>MHHHHHHEPLILTAAITGAETTRADQPNLPITPEEQAKEAKACFEAGARVIHLHIREDDGRPSQRLDRFQEAISAIREVVPEIIIQISTGGAVGESFDKRLAPLALKPEMA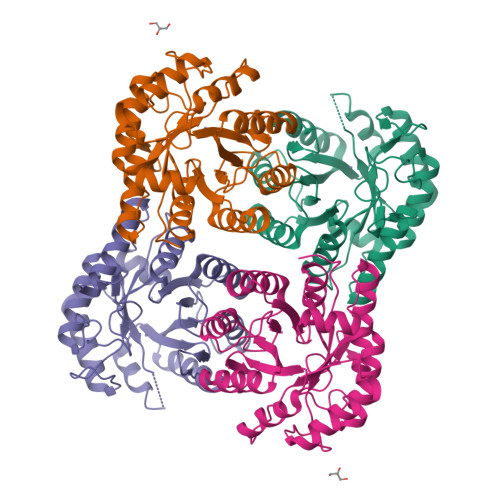TLNAGTLNFGDDIFINHPADIIRLAEAFKQYNVVPEVEVYESGMVDAVARLIKKGIITQNPLHIQFVLGVPGGMSGKPKNLMYMMEHLKEEIPTATWAVAGIGRWHIPTSLIAMVTGGHIRCGFEDNIFYHKGVIAESNAQLVARLARIAKEIGRPLATPEQAREILALNK[4x]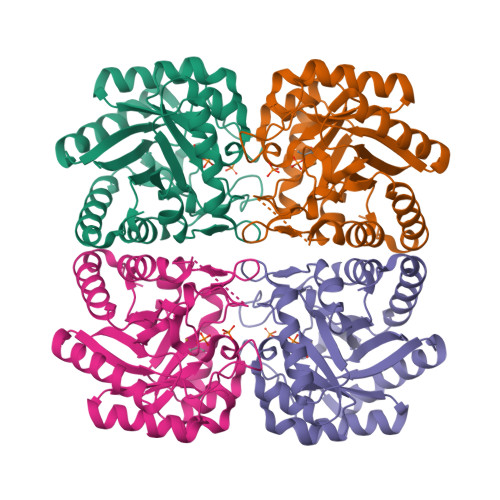>MEKFLVIAGPCAIESEELLLKVGEEIKRLSEKFKEVEFVFKSSFDKANRSSIHSFRGHGLEYGVKALRKVKEEFGLKITTDIHESWQAEPVAEVADIIQIPAFLCRQTDLLLAAAKTGRAVNVKKGQFLAPWDTKNVVEKLKFGGAKEIYLTERGTTFGYNNLVVDFRSLPIMKQWAKVIYDATHSVQLPGGLGDKSGGMREFIFPLIRAAVAVGCDGVFMETHPEPEKALSDASTQLPLSQLEGIIEAILEIREVASKYYETIPVK[2x]>MKFLKNVLEEGSKLEEFNELELSPEDKELLEYLQQTKAKITVVGCGGAGNNTITRLKMEGIEGAKTVAINTDAQQLIRTKADKKILIGKKLTRGLGAGGNPKIGEEAAKESAEEIKAAIQDSDMVFITCGLGGGTGTGSAPVVAEISKKIGALTVAVVTLPFVMEGKVRMKNAMEGLERLKQHTDTLVVIP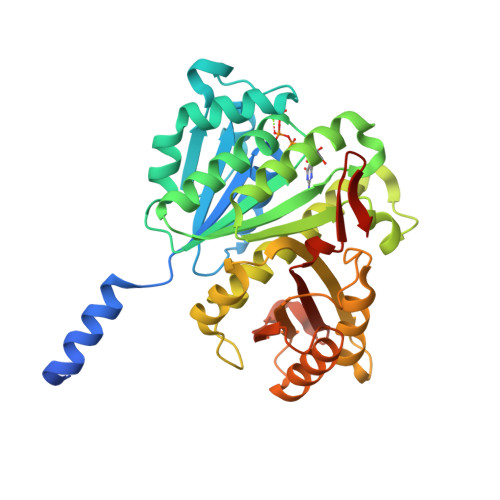NEKLFEIVPNMPLKLAFKVADEVLINAVKGLVELITKDGLINVDFADVKAVMNNGGLAMIGIGESDSEKRAKEAVSMALNSPLLDVDIDGATGALIHVMGPEDLTLEEAREVVATVSSRLDPNATIIWGATIDENLENTVRVLLVITGVQSRIEFTDTGLKRKKLELTGIPKI[2x]Interestingly, DmCE1B in the D. mossii PUL 17 comprises two individual CE1 catalytic domains separated by a small CBM48 domain. To assess the role of each catalytic domain of the multicatalytic DmCE1B, the separate domains were also produced: DmCE1B_nt (45.3 kDa), comprising the N-terminal CE1 domain and the CBM48 domain, and DmCE1B_ct (43.3 kDa) comprising the CBM48 domain and the C-terminal CE1 domain. DmCE1B_ct forms two discrete globular domains, a ten-stranded β-sandwich domain consistent with the CBM48 family structure (residues 294–393) connected via a short linker (residues 394–404) to a three-layer αβα-sandwich (residues 405–656) typical of CE1 enzymes. Comparison to other CE1 family members enables annotation of the catalytic triad in DmCE1B_ct (Ser542, His638, Glu606), which is found in a groove between the CE1 and CBM48 domains.

To investigate potential ligand binding in DmCE1B_ct, we pursued a protein–ligand complex by soaking crystals with methyl ferulate (MFA). We determined the structure of the protein in a different crystal form, which yielded the same dimer interface observed in the apo structure, except for the addition of a partially occupied disulfide bond observed between the two Cys372 residues of each protomer along the noncrystallographic symmetry operator. This disulfide bridge was absent in the structure of the apo protein, which was crystallized at a lower pH (pH 5 versus pH 8 for the complex) but may be biologically relevant to stabilize the dimer formation. Two MFA molecules were observed and modeled: one at the interface between the two CE1 domains of the dimer, and the other close to the active site in one of the protomers. The MFA bound between the two protomers, which is far from either active site and makes minimal interactions with protein, is likely an artifact and not of biological relevance. The second MFA molecule is found on the edge of the active site groove positioned with its methyl ester ∼5 Å from the proposed catalytic center between the catalytic serine and the oxyanion hole. The MFA in DmCE1B_ct makes no direct electrostatic interactions with the protein and is not positioned in line for catalytic cleavage. This is not greatly surprising since the enzyme lacked appreciable activity on MFA. In DmCE1B_ct, the positioning of MFA further away from the catalytic center is possibly due to the smaller loop corresponding to the β-clamp or helical region.

>MGSSHHHHHHSSENLYFQGHSEEAEVGISASTNIPGAQYPQILSGNRVLFRIKAPDAKRVQVDLGKKYDMVREEEGSWAITTDPIVEGFHYYSILIDGVAVCDPASRTFYGMSRMASGIEIPEEGVDYYNLKNVPHGQIRQIRYFSDVTKAWRRAFVYTPAGYDANTSQRYPVLYLQHGGGEDETGWPNQGKMDAIIDNLIAEGKAKPMIVVMDNGYAVDPSASSANSPQGLRGLFQNSALEKVFINEIIPLVDKEFRTIADRDHRAMAGLSMGGFQAFQIAMTNLDKFAYVGGFSGGGIIEQGGDFSKMYNNVWSDVDTFNKRVKLIYLSIGTAEPTNMYQTVNNFHKEFEKAGIKHVYYESPGTSHEWLTWRRSLNQFAELLFK[2x]> GSMEVLKNIRIYPLSNFITSTKNYINLPNELRNLISEEQESKLGFLHIIESDFKPSVALQKLVNCTTGDEKILIIDIVSIWSQQKQRQHGAIYMNSLSCINITGLIVFLELL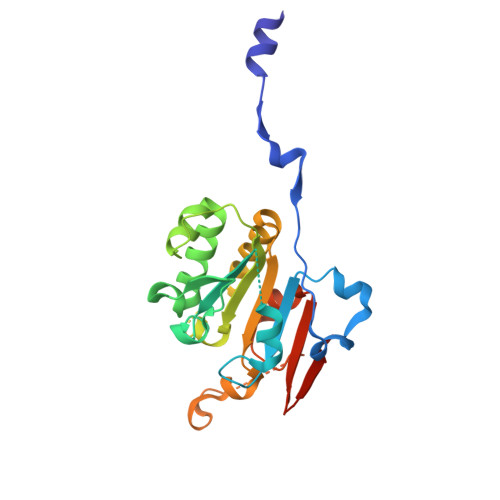YDSPMDALRRCQVDNFNFQLRGIVIDNLSFLNFESDKNYDVINLSKFEKLFKILRKLREFLGCWIITKSFPTDFYNGIENTLVDKWSIKRKSGVTLYPTKLPDSYMKGMDLIIYREVVDGRPQYRRIAALEE>[4x]AEA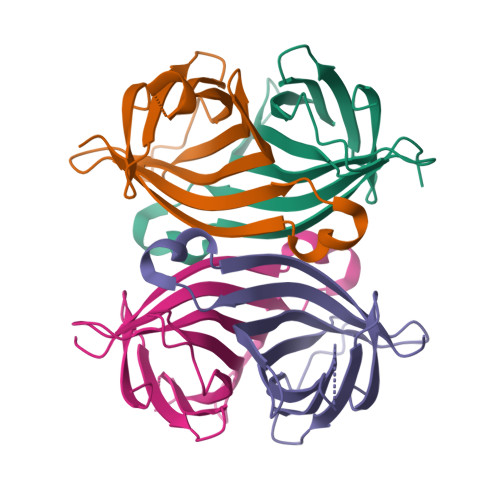GITGTWYEQLGSTFIVTAGADGALTGTYESAVGNAESRYVLTGRYDSAPATDGSGTALGWTVAWKNNYRNAHSATTWSGQYVGGAEARINTQWLLTSGTTEANAWKSTLVGHDTFTKVKPSAAS> GPHMTRHPLQNRWALWYLKADRNKEWEDCLKMVSLFDTVEDFWSLYNHIQSAGGLNWGSDYYLFKEGIKPMWEDVNNVQGGRWLVVVDKQKLQRRTQLLDHYW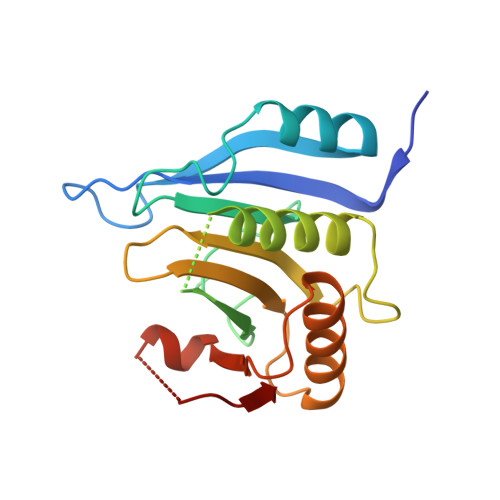LELLMAIVGEQFDEYGDYICGAVVNVRQKGDKVSLWTRDATRDDVNLRIGQVLKQKLSIPDTEILRYEVHKDSSARTSSTVKPRICL> MKRRFTLLGSVVALALSSTALASDAPASRGCADDAGWNDPAMPLKVYGNTWYVGTCGISALLVTSDAGHILVDAATPQAGPQILANIRALGFRPEDVRAIVFSHEHFDHAGSLAELQKATGAPVYARAPAIDTLKRGLPDRTDPAFEVAEPVAPVANIVTLADDGVVSVGPLALTAVASPGHTPGGTSWTWRSCEGDDCRQMVYADSLTAISDDVFRYSDDAAHPGYLAAFRNTLARVAALDCDILVTPHPSASGLWNRIGPRAAAPLMDTTACRRYAQGARQRLEKRLAEEA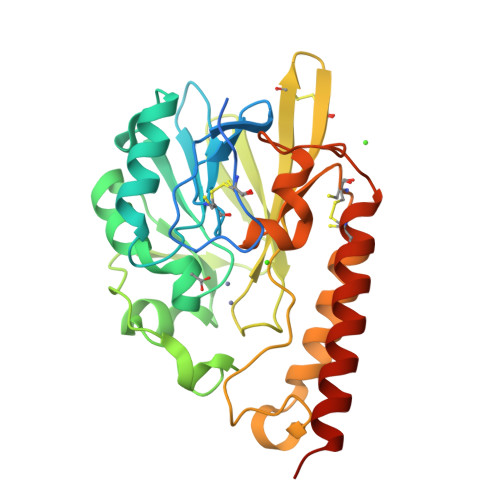ATSPSSGARP In Gram-negative bacteria eﬄux pumps are multimers of three different proteins that form a long transmembrane scaffold linking the cytoplasm to the outside of the cell. These tripartite assemblies are composed of an inner membrane protein from the RND (Resistance Nodulation cell Division) family, which corresponds to the pumping motor that uses the proton-gradient as an energy source; an outer membrane channel from the OMF (Outer Membrane Factor) family; and a periplasmic protein from the MFP (membrane fusion protein) family, anchored to the inner membrane and connecting the other two proteins. In P. aeruginosa, up to 12 different pumps have been sequenced, including OprMOMF-MexAMFP-MexBRND which is one of the most studied pumps because of its constitutive expression whereas the others appear under antibiotic pressure. This study will focus on the versatile membrane channel OprM, which has the ability to work with at least four different pumps, including OprM-MexAB, OprM-MexXY, OprM-MexJK, and OprM-MexMN. The architecture of OprM is composed of a beta-barrel domain that is ∼40 Å in height spanning the outer membrane and a periplasmic alpha-helical domain that is ∼100 Å in length and bears a central buoy. In this study, we have shown that OprM is palmitylated at its N-terminal cysteine by thio-palmitoylation.

To investigate the lipoyl structure, we decided to solve the structure of the best diffracting dataset limited to 3.8 Å resolution. The here-solved structure comprises two trimers in the asymmetric unit with the second trimer being poorly defined. The crystal packing of our C2 OprM structure is slightly different from the P212121 structure but they share common type I crystal packing in which the homo-trimer channels interact in a head-to-head manner through the hydrophobic beta-barrel domains mimicking a lipid bilayer plane. In contrast, when stabilized by a more packed environment around the N-terminus, the entire fatty acid chain appears in the density map of the C2 form where two different orientations are observed. For the three N-termini, the main chain is stabilized by hydrogen bonds with R133 and the carboxyl group of L128. In each case, the palmitoyl tail then turns around two hydrophobic residues, L128 and F129. The palmitoyl from the B monomer (subsequently called Palm-B) is located near the Palm-C of a symmetrical molecule but not close enough to form van der Waals contact because the distance between them is greater than 7 Å. Interestingly, Palm-A instead makes short van der Waals contacts with its own symmetric structure, justifying the quality of the electron density map for this region even at low resolution. The quality of the electron density for this particular monomer makes us confident about the exact nature of the fatty acid modification of OprM.

>[6x]CSLIPDYQRPEAPVAAAYPQGQAYGQNTGAAAVPAADIGWREFFRDPQLQQLIGVALENNRDLRVAALNVEAFRAQYRIQRADLFPRIGVDGSGTRQRLPGDLSTTGSPAISSQYGVTLGTTAWELDLFGRLRSLRDQALEQYLATEQAQRSAQTTLVASVATAYLTLKADQAQLQLTKDTLGTYQKSFDLTQRSYDVGVASALDLRQAQTAVEGARATLAQYTRLVAQDQNALVLLLGSGIPANLPQGLGLDQTLLTEVPAGLPSDLLQRRPDILEAEHQLMAANASIGAARAAFFPSISLTANAGTMSRQLSGLFDAGSGSWLFQPSINLPIFTAGSLRASLDYAKIQKDINVAQYEKAIQTAFQEVADGLAARGTFTEQLQAQRDLVKASDEYYQLADKRYRTGVDNYLTLLDAQRSLFTAQQQLITDRLNQLTSEVNLYKALGGGWNQQTVTQQQTAKKEDPQAHHHHHH> VDLRTLAYSQQQQEKIKPKVRSTVAQHHEALVAHAFTHAHIVALSQHPAALATVAVKYQDMIAALPEATHEAIVAVAKQWSGARALEALLTVAGELRGPPLQLDTGQLLKIAKRGGVTAVEAVHAWRNALTGAPLNLTPEQVVAIASHDGGKQALETVQRLLPVLCQAHGLTPQQVVAIASNGGGKQALETVQRLLPVLCQAHGLTPEQVVAIASNIGGKQALETVQALLPVLCQAHGLTPQQVVAIASNGGGKQALETVQRLLPVLCQAHGLTPEQVVAIASNIGGKQALETVQALLPVLCQAHGLTPEQVVAIASNIGGKQALETVQALLPVLCQAHGLTPEQVVAIASNIGGKQALETVQALLPVLCQAHGLTPEQVVAIASHDGGKQALETVQRLLPVLCQAHGLTPEQVVAIASHDGGKQALETVQRLLPVLCQAHGLTPQQVVAIASNGGGKQALETVQRLLPVLCQAHGLTPEQVVAIASNIGGKQALETVQALLPVLCQAHGLTPEQVVAIASNIGGKQALETVQALLPVLCQAHGLTPEQVVAIASHDGGKQALETVQRLLPVLCQAHGLTPEQVVAIASHDGGKQALETVQRLL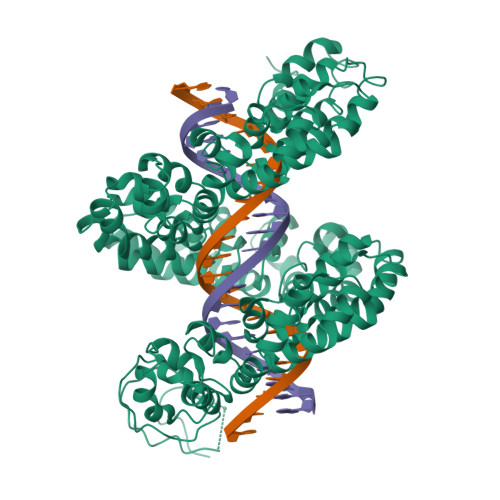PVLCQAHGLTPEQVVAIASHDGGKQALETVQRLLPVLCQAHGLTPQQVVAIASNGGGKQALETVQRLLPVLCQAAGLTPEQVVAIASHDGGKQALETVQRLLPVLCQAHGLTPQQVVAIASNGGGRPALESIVAQLSRPDPGSSAALEHHHHHH> DGVPAVVDCDVHAVLPSPHSLIPYLDEYWADQLVAQLAPTYEPNYHPRGSAIAQHSDASVDENGRAATTAENLVKDVFADGFTDFAVVNCLYGVQQIHQPRREMAHARALNHWIANEWLDKDDRLRASIVVPQGSPRAAAEE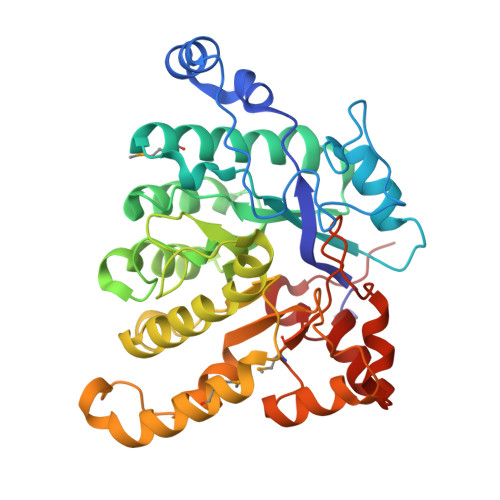IDFWSGDKRFVQVLLLGQSELLYGREINWPIWEAAEAAGLPVTLHIGGVFRQAPTSVGWPASHLEWYVGQQSNIEAQLNSIISEGILQKFPKTKILLSELGFNWLPPFMWKFDKLWKSYRPDIPWVQESPLELIREHVRVTTSPSDGAEEAGRLDSIVDRLGSDRMLVYSSDYPHKHHSGPRDIENGTHSPELLDRIYRRNAFDLYNLVVPS The obtained experimental data revealed that triazoles induced the aggregation of Thermoanaerobacter brockii alcohol dehydrogenase (TbSADH) to form a gel complex; however, its stability was very low. Intermolecular interactions in this gel were strengthened by the synergistic chelation of metal ions. The active center catalyzing the asymmetric reduction of aryl prochiral ketones is mainly composed of Zn2+ ions and three amino acid residues (H59, C37, and D150). The activity of TbSADH is associated with the rate of hydride transfer from NADPH to the substrate.

Using cryogenic electron microscopy (Cryo-EM), a structure–property relationship of the enzyme after gelation was analyzed for the improved catalytic performance, and a near-atomic-level enzyme structure with an ultra-high resolution of 2.1 Å was obtained. In this model, the tetrameric enzyme has a symmetrical tetrahedral structure with one Zn2+ active center in each subunit, and no Hmtz was found in the structure, suggesting that Hmtz may bind to the enzyme by a non-specific manner. According to the structure of the active center, Zn2+ was not bound by triazole, indicating that the triazoles acted on the enzyme surface without entering the active center to scavenge Zn2+. Moreover, the cryo-EM structure of EAG enzyme provides a structural perspective for its activity enhancement. The large motion of the loop consisting of residues L107 to H100 with a 4.1 Å shift at residue L107 and 10.5 Å shift at residue H100 leads to a major structural rearrangement of the mutant. The loop motion further induced the side chain flipping of residue W110 with a torsion angle of 94.5°, thereby expanding the substrate-binding pocket of the enzyme. The larger binding pocket may promote the conformational sampling of the substrate and increase the frequency of productive binding modes, thereby increasing the catalytic efficiency of the enzyme. This is consistent with the increased kcat value obtained using a kinetic analysis. Meanwhile, the coordination effect of Mg2+ ions improved the enzyme robustness, which resulted in higher stability than that of the free enzyme against various unfavorable environmental factors. Note that in the presence of trypsin (3 mg mL−1 for 3 h at 25 °C), EAG retained 74.6% of its original activity compared to the value of 15.3% determined for the free enzyme. In addition, the melting temperature (Tm) of EAG (10 mM Mg2+) measured using differential scanning calorimetry (DSC) was 133.8 °C, which was 35.2 °C higher than that of the free enzyme (see below), indicating that the robustness of EAG was significantly improved with respect to that of the free enzyme.

>[4x]MHHHHHHKGFAMLSIGKVGWIEKEKPAPGPFDAIVRPLAVAPCTSDIHTVFEGAIGERHNMILGHEAVGEVVEVGSEVKDFKPGDRVVVPANTPDWRTSEVQRGYHQHSGGMLAGWKFSNVKDGVFGEFFHVNDADMNLAHLPKEIPLEAAVMIPDMMTTGFHGAELADIELGATVAVLGIGPVGLMAVAGAKLRGAGRIIAVGSRPVCVDAAKYYGATDIVNYKDGPIESQIMNLTEGKGVDAAIIAGGNADIMATAVKIVKPGGTIANVNYFGEGEVLPVPRLEWGCGMAHKTIKGGLCPGGRLRMERLIDLVFYKRVDPSKLVTHVFRGFDNIEKAFMLMKDKPKDLIKPVVILA>[2x]MRIIMPVEFSRIVRDVERLIAVEKYSLQGVVDGDKLLVVGFSEGSVNAYLYDGGETVKLNREPINSVLDPHYGVGRVILVRDVSKGAEQHALFKVNTSRPGEEQRLEAVKPMRILSGVDTGEAVVFTGATEDRVALYALDGGGLRELARLPGFGFVSDIRGDLIAGLGFFGGGRVSLFTSNLSSGGLRVFDSGEGSFSSASISPGMKVTAGLETAREARLVTVDPRDGSVEDLELPSKDFSSYRPTAITWLGYLPDGRLAVVARREGRSAVFIDGERVEAPQGNHGRVVLWRGKLVTSHTSLSTPPRIVSLPSGEPLLEGGLPEDLRRSIAGSRLVW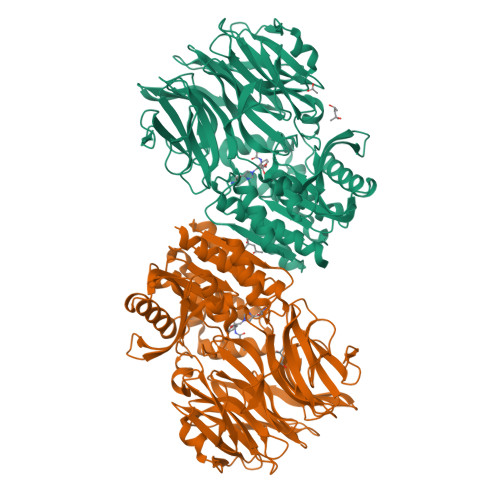VESFDGSRVPTYVLESGRAPTPGPTVVLVHGGPFAEDSDSWDTFAASLAAAGFHVVMPNYRGSTGYGEEWRLKIIGDPCGGELEDVSAAARWARESGLASELYIMGYSYGGYMTLCALTMKPGLFKAGVAGASVVDWEEMYELSDAAFRNFIEQLTGGSREIMRSRSPINHVDRIKEPLALIHPQNDSRTPLKPLLRLMGELLARGKTFEAHIIPDAGHAINTMEDAVKILLPAVFFLATQRERR> LPPKPEE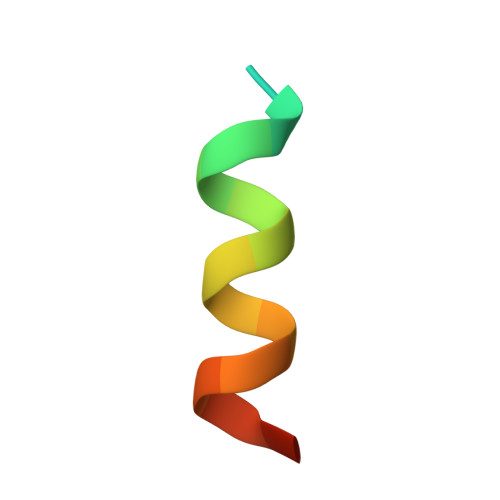RWRYIKELESRQ>[2x]MAACRALKAVLVDLSGTLHIEDAAVPGAQEALKRLRGASVIIRFVTNTTKESKQDLLER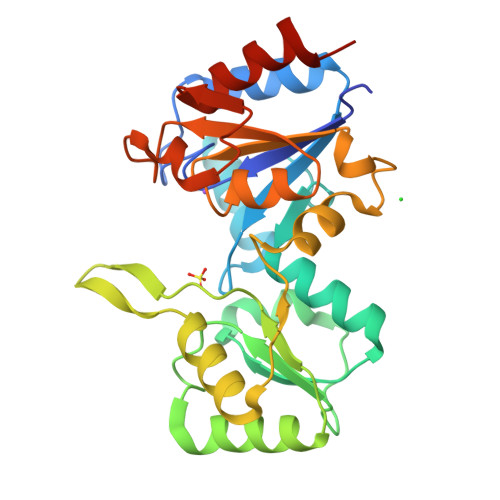LRKLEFDISEDEIFTSLTAARSLLERKQVRPMLLVDDRALPDFKGIQTSDPNAVVMGLAPEHFHYQILNQAFRLLLDGAPLIAIHKARYYKRKDGLALGPGPFVTALEYATDTKATVVGKPEKTFFLEALRGTGCEPEEAVMIGDDCRDDVGGAQDVGMLGILVKTGKYRASDEEKINPPPYLTCESFPHAVDHILQHLLAENLYFQ>[2x]EFRAPLASPPNSSYIDWRTFKGNGVNLGGWLEQESTIDSLFWDKYSGGASDEWGLCEHLGSQCGPVLEHRYATLITKADIDKLASGGITVLRIPTTYAAWIDLPSSQLYSGNQTAYLKEIADYAIKTYNMHIIIDTHSLPGGVNGLTIGEATGHWYWFYNETHFNYSMQVIDQVINFIQTSGSPQSYTLEPINEPADNNTNMVVFGTPLALTDHGAAWVLKYIRAVVQRVESVNPNIPVMFQ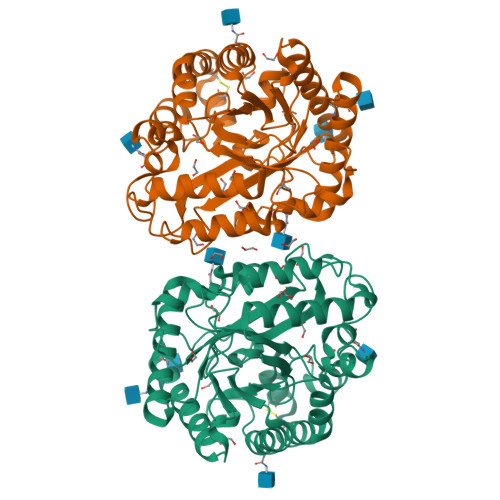GSFKYPQYWEGDFPASTNLVFDTHHYYYEHMDSSSENLPEYILADAREKSGTGKFPVFVGEWAIQATYNNTLALRKRNVLAGLETWSSFSQGSSYWTAKFTGNTSVAGQGEQKDYWCYETFIDEGYFN Aromatic residues cluster in the core of folded proteins, where they stabilize the structure through multiple interactions. NMR studies in the 1970s demonstrated that aromatic side chains can undergo ring flips—that is, 180° rotations of the χ2 dihedral angle (Cβ–Cγ axis)—even when engaged in stabilizing interactions in the hydrophobic core. Here we capture ring flipping events of a buried tyrosine residue in the SH3 domain of the JNK-interacting protein 1 (JIP1). Our data therefore suggest that the conformation of the aromatic ring at position 526 is determined by steric interactions dictated by the size of the surrounding amino acids.

The data confirm that exchange contributions to the transverse relaxation are present for residues within three regions of the protein. These residues are located spatially close to tyrosine 526 (Y526). A mutation of Y526 to alanine (Y526A) shows no conformational exchange, and conserves the protein backbone conformation, as evidenced from its crystal structure that we obtained at 1.5-Å resolution. These results show that the relaxation dispersion that affects around 40% of the residues in the SH3 domain arises from a single exchange process, with Y526 being the origin of the observed exchange.

>[12x]GHMEQTHRAIFRFVPRHEDELELEVDDPLLVELQAEDYWAEAYNMRTGARGVFPAYYAIEVTK>[6x]RSRIFKIIVIGDSNVGKTCLTYRFCAGRFPDRTEATIGVDFRERAVDIDGERIKIQLWDTAGLERFRKSMVQHYYRNVHAVVFVYDMTNMASFHSLPAWIEECKQHLLANDIPRILVGNKCDLRSAIQVPTDLAQKFADTHSMPLFETSAKNPNDNDHVEAIFMTLAHKLKSH;>DLEVANQTLKDEYDALQITFTALEEKLRKTTEENQELVTRWMAEKAQEANRLNAENE[6x]

The Atg12-Atg5/Atg16 complex has E3 ligase activity towards Atg8 and LC3 lipidation. Rab proteins are key regulators of intracellular membrane trafficking processes and are also involved in the formation and maturation of autophagosomes and their fusion with lysosomes. Rab33B interacts with Atg16L1 in a GTP dependent manner and therefore Atg16L1 is an effector of Rab33B. The interaction between Atg16L1 and Rab33B might facilitate the recruitment of Golgi derived vesicles to the growing isolation membrane.

Since Atg16L1 is an effector of Rab33B, the GTPase deficient Rab33B(30–202) Q92L mutant was used to stabilize the Rab33B/Atg16L1 complexes. The crystal structure of the Atg16L1(153–210)/Rab33B Q92L complex was determined at 3.47 Å resolution. The Rab33B/Atg16 complex is a heterotetramer and the model comprises an Atg16L1 coiled-coil dimer and two Rab33B molecules. The two mRab33B molecules bind to the diverging C-terminal ends of the coiled-coil and are not in direct contact. There are three Rab33B/Atg16L1 complexes in the asymmetric unit, which align with a root-mean-square deviation (RMSD) of 0.60 Å. The N-terminal end of Atg16L1 is positioned in the proximity of the opposing Rab33B molecule, and residues E186 of the Atg16L1 dimer form salt bridges with nearby positioned Rab33B R94 residues localized in switch II, while hydrogen bonds between R193 of the Atg16L1 dimer and the carbonyl oxygens of Rab33B A64 in switch I are formed. The diverging Atg16L1 helices then interact with switch I, switch II and the interswitch regions of the nearby Rab33B molecule through hydrophobic interactions and a salt bridge between Atg16L1 K198 and Rab33B D69. At the C-terminal end, the Rab33B aromatic triad, composed of residues F70, W87 and Y103, forms hydrophobic interactions with Atg16L1. The structures of Atg16L1 bound Rab33B and free GppNHp-bound Rab33B 34 are very similar with the exception of the F70 side chain, which adopts a different conformation to accommodate Atg16L1 binding. The Atg16L1 helices start diverging from residue 189 onwards due the large side chain of W194 and W194′ facing each other at the coiled-coil core and repulsive electrostatic interactions between E197 and E197′ and E201 and E201′ from the two α-helices.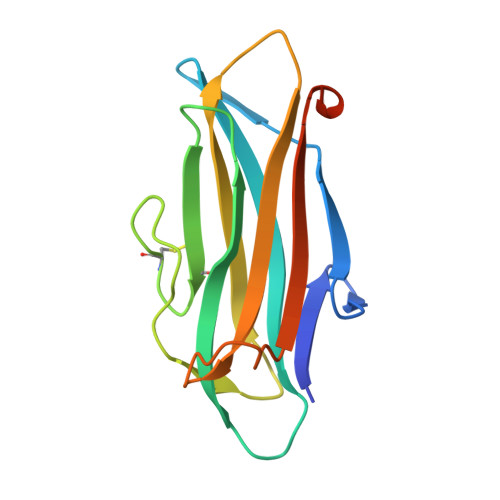> GSHQVVIKVGDAILENNATVDITAFTTEDGTEEMKFKGMVINQSATPINVIGKITKQEMIGDGHFALCFGQCMLPNVSVSPVVEVGGEGEPLSLRYTFPVSNEGHTGAFTFSCFPESGAPGTELATVNINFKYKGGGTDLTNIGLGR> DEEEEDGTMKRNATSPQVQR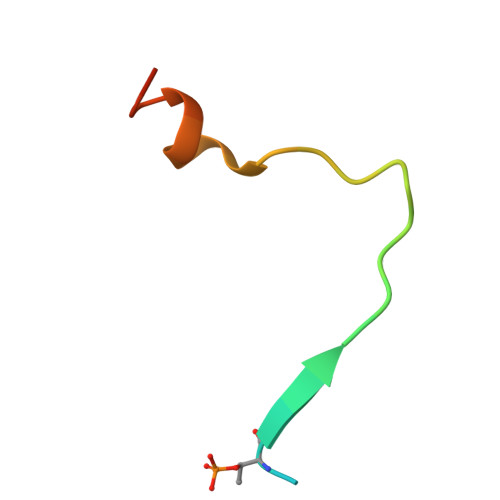PSFMDYFDKQD>[12x]SNAMAGNFANARVEKLIRQAGAQRVSADAVDKMNEILTDW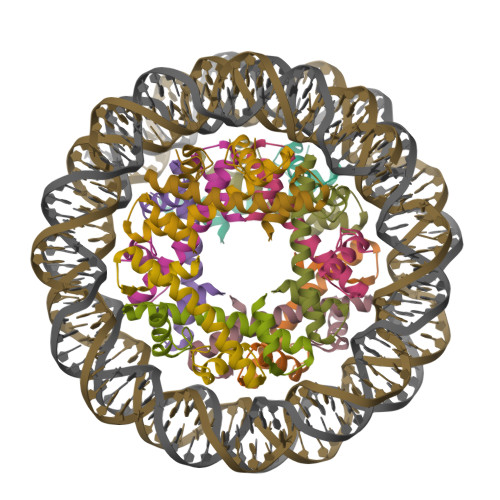GKNIAKYAVEIARHSGRKTVKENDIKLAAQK>[2x]MSTTTTEARSPLPLLLRRGRSSTALSASTAEARSPLSILQFRRRSSKDVRNITSVSSSLLPAFGTFIEDDNPSSKPFIVLHFDRRYRLWELFLVILVGYSAWASLFELAFEKAAEGALLTIDLVVDFFFAVDIILTFFVSYLDNTTYLNVTDHKLIAKRYLKSVAFVMDVASTLPIQFIYKTITGDVGRGQAFGFLNLLRLWRLRRVAELFKRLEKDAHFNYFVIRVIKLLCVTIFWIHLAGCILYWIAYHYPRPTDTWIGSQVEDFKERSVWLGYTYSMYWSIVTLTTVGYGDLHAVNSREKTFNMFYMLFNIGLTSYIIGIMTNLVVHGALRTFAMRSAINDILRYTSKNRLPDTMREQMLAHMQLKFKTAELRQEEVLQDLPKAIRSSINQHLFRSIIEEAYLFKGFPEGLLVQLVSQIQAEYFPPKMEIILQNEIPTDFYVIVSGGVDIIASKGVSEQVLAKLGPGSMAGEIGVVFNIPQPFTVRTRRLSQVIRIGHHKFKEMVQSDNDVDAKMIIANFMTYLKGLNDELKKEIPFLRDLLDDADAQVQETVQSEETPQSNDEEIVTVSRHENGQIEERRREGVPKRVIIHGQAPPNQDNKNNGDSNGRLIILPDSIQLLFDLAEKKLGKRGST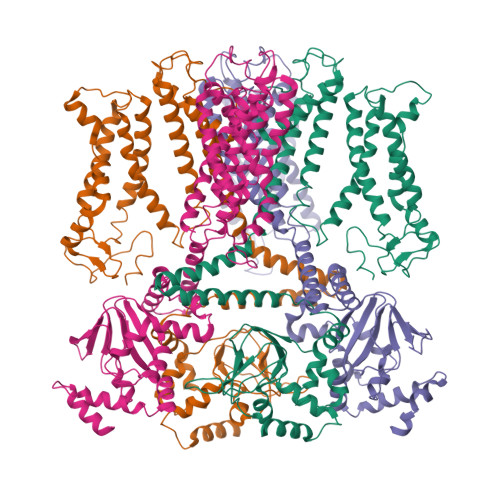IAMADGAHVEQIDALRENDHLYIF;>MRGGALLCGQVQDEIEQLSRESSHFSLSTGILPSLGARSNRRVKLRRFVVSPYDHKYRIWEAFLVVLVVYTAWVSPFEFGFLRKPRPPLSITDNIVNAFFAIDIIMTFFVGYLDKSTYLIVDDRKQIAFKYLRSWFLLDLVSTIPSEAAMRISSQSYGLFNMLRLWRLRRVGALFARLEKDRNFNYFWVRCAKLVCVTLFAVHCAACFYYLIAARNSNPAKTWIGANVANFLEESLWMRYVTSMYWSITTLTTVGYGDLHPVNTKEMIFDIFYMLFNLGLTAYLIGNMTNLVVHGTSRTRNFRDTIQAASNFAHRNHLPPRLQDQMLAHLCLKYRTDSEGLQQQETLDALPKAIRSSISHFLFYSLMDKVYLFRGVSNDLLFQLVSEMKAEYFPPKEDVILQNEAPTDFYILVNGTADLVDVDTGTESIVREVKAGDIIGEIGVLCYRPQLFTVRTKRLCQLLRMNRTTFLNIIQANVGDGTIIMNNLLQHLKEMNDPVMTNVLLEIENMLARGKMDLPLNLCFAAIREDDLLLHQLLKRGLDPNESDNNGRTPLHIAASKGTLNCVLLLLEYHADPNCRDAEGSVPLWEAMVEGHEKVVKVLLEHGSTIDAGDVGHFACTAAEQGNLKLLKEIVLHGGDVTRPRATGTSALHTAVCEENIEMVKYLLEQGADVNKQDMHGWTPRDLAEQQGHEDIKALFREKLHERRVHIETSSSVPILKTGIRFLGRFTSEPNIRPASREVSFRIRETRARRKTNNFDNSLFGILANQSVPKNGLATVDEGRTGNPVRVTISCAEKDDIAGKLVLLPGSFKELLELGSNKFGIVATKVMNKDNNAEIDDVDVIRDGDHLIFATDS[2x]However, analyses of the formation of TF complexes on DNA have revealed that many TFs also bind together across the family boundaries, in a DNA-dependent or DNA-facilitated manner. Because the DNA-bound TFs are fixed at particular positions relative to each other, the contact surfaces required for cooperative DNA-facilitated binding are very small, and can evolve rapidly. We also generated an unseen test set by solving six structures that represent several TF–TF–DNA complexes bound to optimal DNA sequences. The structures included two BARHL2 homodimers with two spacings, HOXB13 homodimer and TEAD4–HOXB13, MEIS1–HOXB13 and FOXK1–ELF1 heterodimers.

Recently released versions of RoseTTAFold (RoseTTAFold2NA v.0.2)39 and AlphaFold (AlphaFold v.3.0), which can predict the structures of protein–nucleic acid complexes, performed much better in predicting the overall geometry of TF–TF–DNA complexes. For example, both RoseTTAFold2NA and AlphaFold 3 correctly predicted the two homodimers of BARHL2. However, they still failed in most cases to correctly predict preferred spacings and orientations of TF–TF pairs bound to DNA, owing potentially to their inability to predict key TF–TF and TF–DNA contacts that depend on the orientation and spacing of the TF pairs.

>[4x]PRKARTAFSDHQLNQLERSFERQKYLSVQDRMDLAAALNLTDTQVKTWYQNRRTKWKRQT>[3x]MAIRFFTILLSTFFLTSFVYAQEHVVIRSDWKKFFSDLQAEGAIVIADERQAKHTLSVFDQERAAKRYSPASTFKIPHTLFALDADAVRDEFQVFRWDGVNRSFAGHNQDQDLRSAMRNSTVWVYELF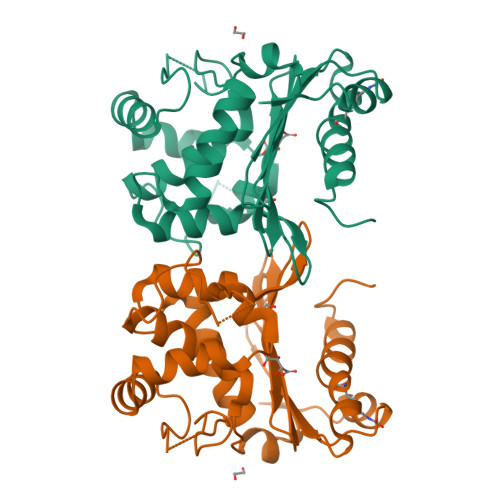AKDIGEDKARRYLKQIDYGNVDPSTIKGDYWIDGNLKISAHEQILFLRKLYRNQLPFKVEHQRLVKDLMITEAGRSWILRAKTGWEGRFGWWVGWIEWPTGPVFFALNIDTPNRTDDLFKREAIARAILRSIDALPPN> MLDDRARMEAAKKEKVEQILAEFQLQEEDLKKVMRRMQKEMDRGLRLETHEEASVKMLPTYVRSTPEGSEVGDFLSLDLGGTNFRVMLVKVGEGEEGQWSVKTKHQMYSIPEDAMTGTAEMLFDYISECISDFLDKHQMKHKKLPLGFTFSFPVRHEDIDKGILLNWTKGFKASGAEGNNVVGLLRDAIKRRGDFEMDVVAMVNDTVATMI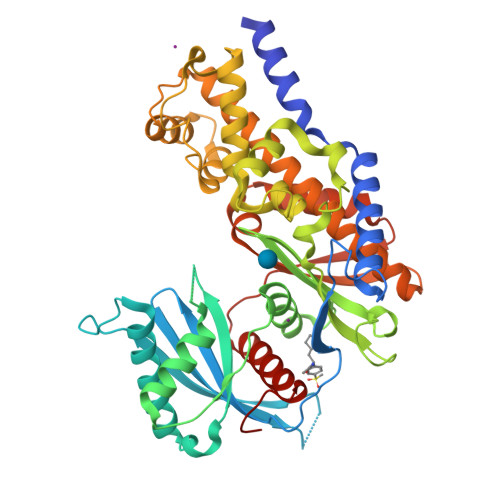SCYYEDHQCEVGMIVGTGCNACYMEEMQNVELVEGDEGRMCVNTEWGAFGDSGELDEFLLEYDRLVDESSANPGQQLYEKLIGGKYMGELVRLVLLRLVDENLLFHGEASEQLRTRGAFETRFVSQVESDTGDRKQIYNILSTLGLRPSTTDCDIVRRACESVSTRAAHMCSAGLAGVINRMRESRSEDVMRITVGVDGSVYKLHPSFKERFHASVRRLTPSCEITFIESEEGSGRGAALVSAVACKKACMLGQLEHHHHHH> RSPVFTDNSSPPAVPQSFQVAHLHAPTGSGKSTKVPAAYAAQGYKVLVLNPSVAATLGFGVYMSKAHGIDPNIRTGVRAITTGGPITYSTYGKFLADGGCSGGAYDIIICDECH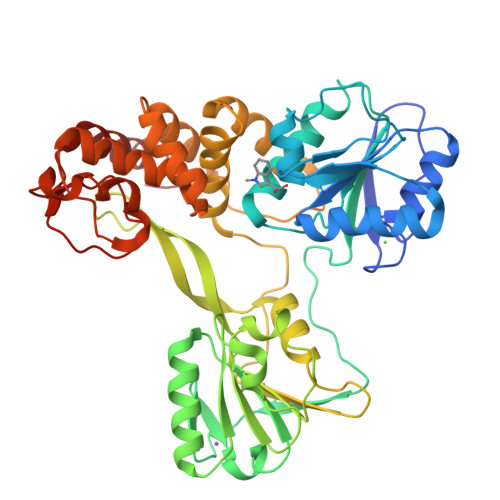STDSTSILGIGTVLDQAETAGARLVVLATATPPGSVTVSHPNIEEVALSNTGEIPFYGKAIPIEVIRGGRHLIFCHSKKKCDELAAKLSALGLNAVAYYRGLDVSVIPTSGDVVVVATDALMTGYTGDFDSVIDCNTCVTQTVDFSLDPTFTIDTTTVPQDAVSRSQRRGRTGRGRRGIYRFVTPGERPSGMFDSSVLCECYDAGCAWYELTPAETSVRLRAYLNTPGLPVCQDHLEFWESVFTGLTHIDAHFLSQTKQAGDNFPYLVAYQATVCARAQAPPPSWDQMWKSLTRLKPTLLGPTPLLYRLGALQNEVTLTHPITKYIMACMSADLEVV>MALVYDAEFVGSEREFEEERETFLKGVKAYDGVLATRYLMERSSSAKNDEELLELHQNFILLTGSYACSIDPTEDRYQNVIVRGVNFDERVQRLSTGGSPARYAIVYRRGWRAIAKALDIDEEDVPAIEVRAVKRNPLQPALYRILVRYGRVDLMPVTVDEVPPEMAGEFERLIERYDVPIDEKEERILEILRENPWTPHDEIARRLGLSVSEVEGEKDPESSGIYSLWSRVVVNIEYDERTAKRHVKRRDRLLEELYEHLEELSERYLRHPLTRRWIVEHKRDIMRRYLEQRIVECALKLQDRYGIREDVALCLARAFDGSISMIATTPYRTLKDVCPDLTLEEAKSVNRTLATLIDEHGLSPDAADELIEHFESIAGILATDLEEIERMYEEGRLSEEAYRAAVEIQLAELTKKEGVGRKTAERLLRAFGNPERVKQLAREFEIEKLASVEGVGERVLRSLVPGYASLISIRGIDRERAERLLKKYGGYSKVREAGVEELREDGLTDAQIRELKGL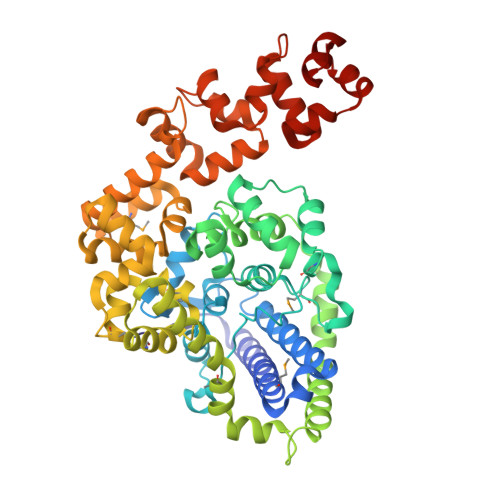K[2x]(3R,5R)-7-[5-(ANILINOCARBONYL)-3,4-BIS(4-FLUOROPHENYL)-1-ISOPROPYL-1H-PYRROL-2-YL]-3,5-DIHYDROXYHEPTANOIC ACID | C33 H34 F2 N2 O5 | 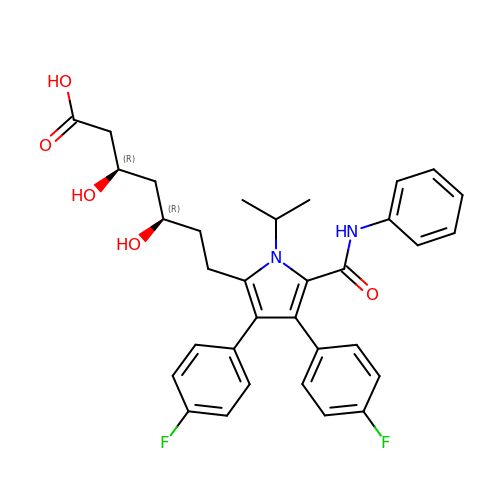VZMMUQFHUUOVEM-KAYWLYCHSA-N> VADRGQRRGCAPGIASALRASFQGKSRPWTQTRYWAFALLTPLVVAMVLTGCSASGTQLELAPTADRRAAVGTTSDINQQDPATLQDGGNLRLSLTDFPPNFNILHIDGNNAEVAAMMKATLPRAFIIGPDGSTTVDTNYFTSIELTRTAPQVVTYTINPEAVWSDGTPITWRDIASQIHAISGADKAFEIASSSGAERVASVTRGVDDRQAVVTFAKPYAEWRGMFAGNGMLLPASMTATPEAFNKGQLDGPGPSAGPFVVSALDRTAQRIVLTRNPRWWGARPRLDSITYLVLDDAARLPALQNNTIDATGVGTLDQLT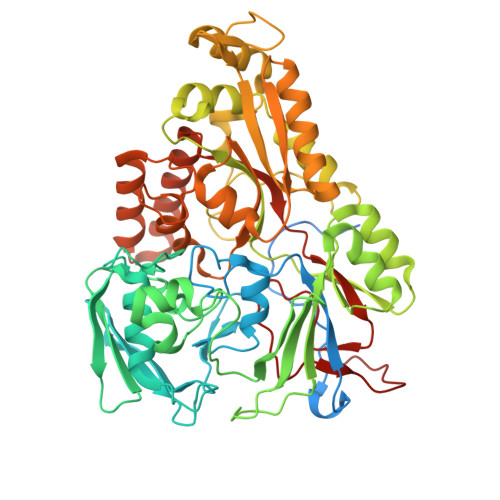IAARTKGISIRRAPGPSWYHFTLNGAPGSILADKALRLAIAKGIDRYTIARVAQYGLTSDPVPLNNHVFVAGQDGYQDNSGVVAYNPEQAKRELDALGWRRSGAFREKDGRQLVIRDLFYDAQSTRQFAQIAQHTLAQIGVKLELQAKSGSGFFSDYVNVGAFDIAQFGWVGDAFPLSSLTQIYASDGESNFGKIGSPQIDAAIERTLAELDPGKARALANQVDELIWAEGFSLPLTQSPGTVAVRSTLANFGATGLADLDYTAIGFMRRHHHHHHHH>MMRWDDKKPIYQQLRDKIVEAIIDGSYVEGEMIPSIRKISTEYQINPLTVSKAYQSLLDDNVIEKRRGLGMLVKAGARQRLLTQEKQYFLKKQWPQIKNKLE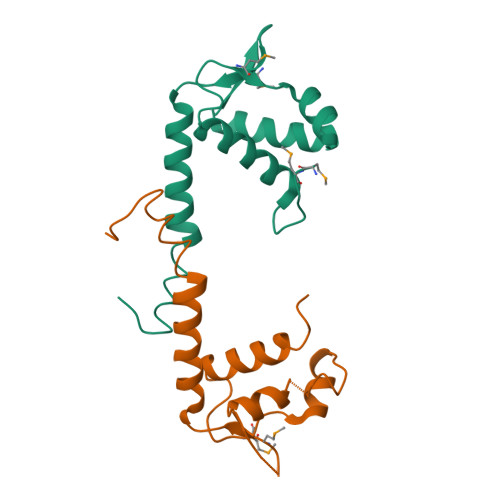RLGIDLKELLK[3x]>MVVLAGPPAVDHIPLLRSPDPGDVFSGVPVVDLGSPGAARAVVDACER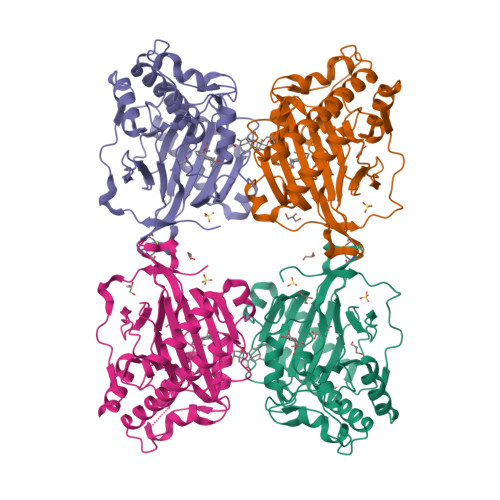YGFFKVVNHGVATDTMDKAESEAVRFFSQTQPDKDRSGPAYPFGYGSKRIGFNGDMGWLEYLLLALDDASLADACTVPSCAVFRAALNEYISGVRKVAVRVMEAMSEGLGIAQADALSALVTAEGSDQVFRVNHYPPCRALQGLGCSVTGFGEHTDPQLVSVLRSNGTSGLQIALRDGQWVSVPSDRDSFFVNVGDSLQVLTNGRFKSVKHRVVANSLKSRVSFIYFGGPPLAQRIAPLPQLLGEGEQSLYKEFTWDEYKKAAYKSRLGDNRLAQFEKK[4x]> MVSQIGLLLPLSGDGQILGTTIQSGFNDAKGNSTIPVQVFDTSMNSVQDIIAQAKQAGIKTLVGPLLKQNLDVILADPAQIQGMDVLALNATPNSRAIPQLCYYGLSPEDEAESAANKMWNDGVRNPLVAMPQNDLGQRVGNAFNVRWQQLAGTDANIRYYNLPADVTYFVQENNSNTTALYAVASPTELAEMKGYLTNIVPNLAIYASSRASASATNTNTDFIAQMNGVQFSDIPFFKDTNSPQYQKLAKSTGGEYQLMRLYAMGADAWLLINQFNELRQVPGYRLSGLTGILSADTNCNVERDMTWYQYQDGA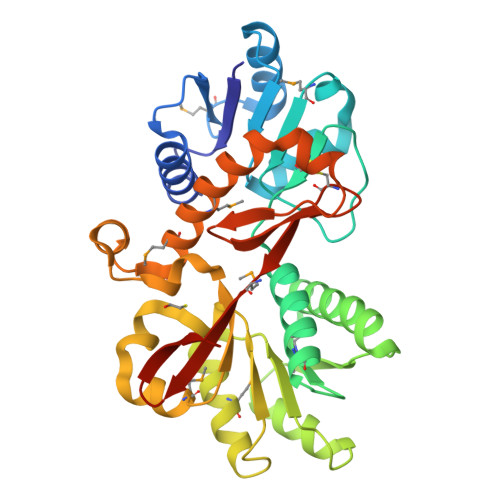IVPVVDHHHHHH>[2x]SGHGMEENGMKSKILIFGGTGYIGNHMVKGSLKLGHPTYVFTRPNSSKTTLLDEFQSLGAIIVKGELDEHEKLVELMKKVDVVISALAFPQILDQFKILEAIKVAGNIKRFLPSDFGVEEDRINALPPFEALIERQRMIRRAIEEANIPYTYVSANCFASYFINYLLRPYDPKDEITVYGTGEAKFAMNYEQDIGLYTIKVATDPRALNRVVIYRPS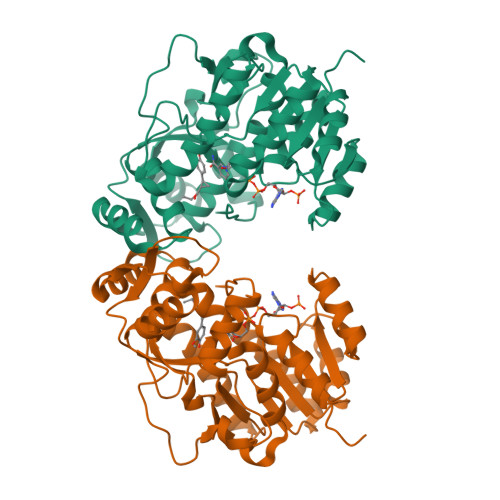TNIITQLELISRWEKKIGKKFKKIHVPEEEIVALTKELPEPENIPIAILHCLFIDGATMSYDFKENDVEASTLYPELKFTTIDELLDIFVHDPPPPASAAF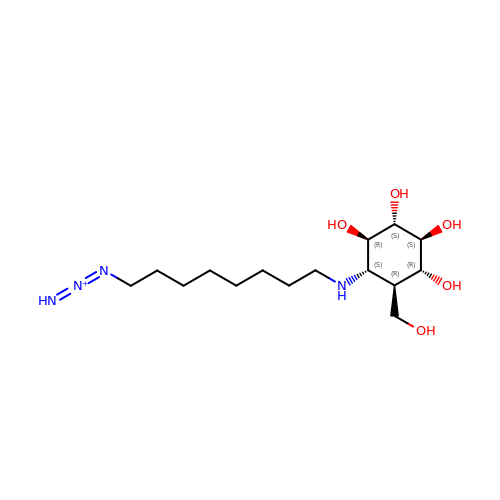1-(8-{[(1S,2R,3S,4S,5R,6R)-2,3,4,5-tetrahydroxy-6-(hydroxymethyl)cyclohexyl]amino}octyl)triaza-1,2-dien-2-ium | C15 H31 N4 O5 | KPTZFIOZQLVZBJ-SAAWNECCSA-N> MADIYPLGKTHTEELNEIIVESAKEIAEPDTTMIQKLIDEHNPEPLLKGVRYYMCENDIEKKRRTYYDAAGQQLVDDTKTNNRTSHAWHKLFVDQKTQYLVGEPVTFTSDNKTLLEYVNELADDDFDDILNETVKNMSNKGIEYWHPFVDEEGEFDYVIFPAEEMIVVYKDNTRRDILFALRYYSYKGIMGEETQKAELYTDTHVYYYEKIDGVYQMDYSYGENNPRPHMTKGGQAIGWGRVPIIPFKNNEEMVSDLKFYKDLIDNYDSITSSTMDSFSDFQQIVYVLKNYDGENPKEFTANLRYHSVIKVSGDGGVDTLRAEIPVDSAAKELERIQDELYKSAQAVDNSPETIGGGATGPALEKLYALLDLKANMAERKIRAGLRLFFWFFAEYLRNTGKGDFNPDKELTMTFTRTRIQNDSEIVQSLVQGVTGGIMSKETAVARNPFVQDPEE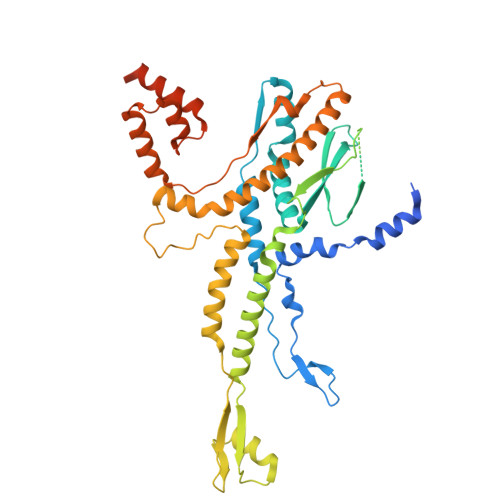ELARIEEEMNQYAEMQGNLLDDEGGDDDLEEDDPNAGAAESGGAGQVS> AYQLYRNTTLGNSLQESLDELIQSQQITPQLALQV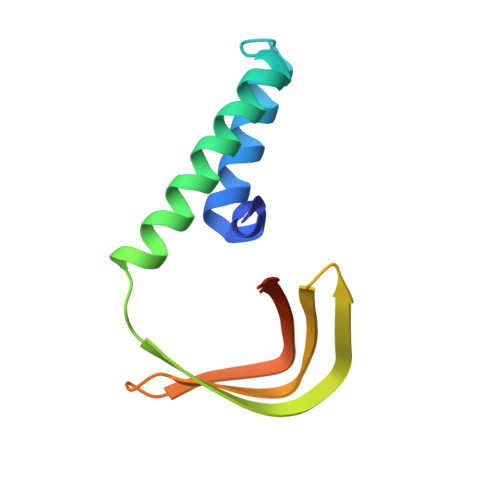LLQFDKAINAALAQRVRNRVNFRGSLNTYRFCDNVWTFVLNDVEFREVTELIKVDKVKIVACDGKNTGSNTTE> DTHSIIQFLQRPVLIDNIEIIAGT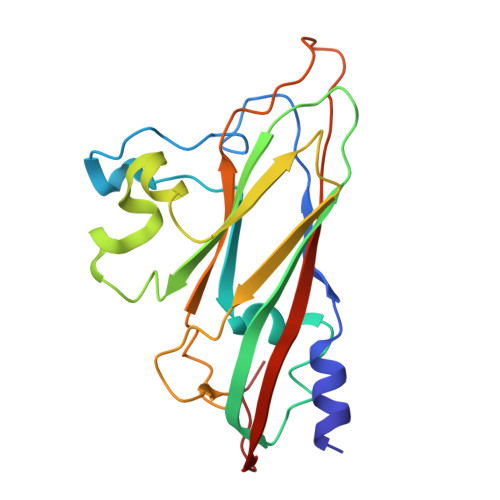TADAAKPLSRYVLDQQNSQKYVRSWTLPSTVLKAGGKAQKLANFKYLRCDVQVKLVLNANPFVAGRMYLAYSPYDDKVDTARSVLQTSRAGVTGYPGVELDFQLDNSVEMTIPYASFQEAYDLVTGTEDFVQLYLFPITPVLGPKSESESSKVDISVYMWLSNISLVIPTYRMNPD>[4x]GSEPAMEPETLEARINRATNPLNKELDWASINGFCEQLNEDFE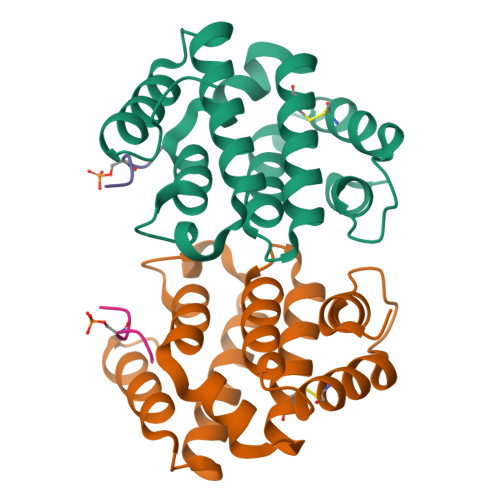GPPLATRLLAHKIQSPQEWEAIQALTVLETCMKSCGKRFHDEVGKFRFLNELIKVVSPKYLGSRTSEKVKNKILELLYSWTVGLPEEVKIAEAYQMLKKQGIVKSDPKLPDDTTF;>ADDISLLK[4x]4-(2-{[(2-amino-4-methylquinolin-7-yl)methyl]amino}ethyl)benzonitrile 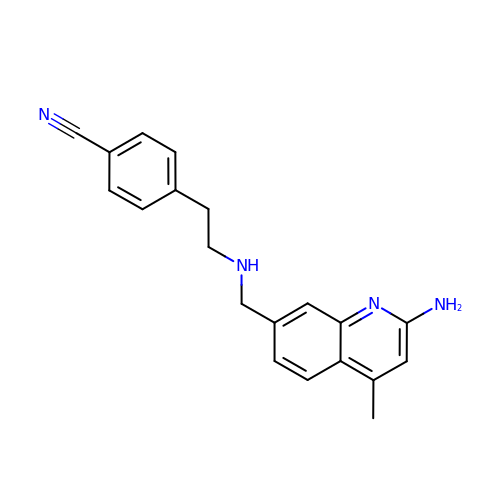| C20 H20 N4 | CNMLPDIDKJDXOA-UHFFFAOYSA-N>[9x]PDVPKGCEGPCKVQSYEQRHDISHVGKVLCVSDVTRGNGLTHRVGKRFCVKSVYVLGKIWMDENIKTKNHTNTVMFYLVRDRRPFGTAMDFGQVFNMYDNEPSTATIKNDLRDRYQVLRKFTSTVTGGQYASKEQALVKKFMKINNYVVYNHQEAAKYDNHTENALLLYMACTHASNPVYATLKIRIYFYDSVQN;> NRR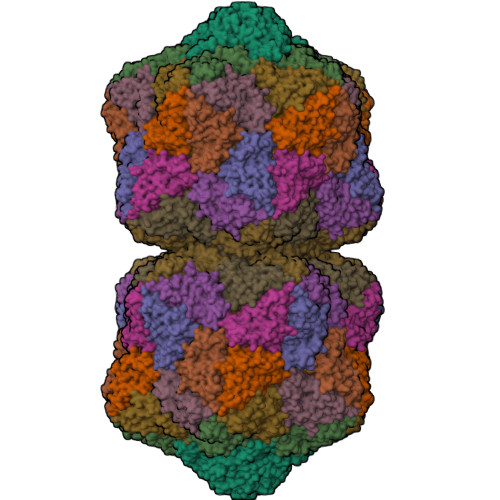RTWTNRPMYRKPRLYRMYRTPDVPKGCEGPCKVQSYEQRHDISHVGKVLCVSDVTRGNGLTHRVGKRFCVKSVYVLGKIWMDENIKTKNHTNTVMFYLVRDRRPFGTAMDFGQVFNMYDNEPSTATIKNDLRDRYQVLRKFTSTVTGGQYASKEQALVKKFMKINNYVVYNHQEAAKYDNHTENALLLYMACTHASNPVYATLKIRIYFYDSVQN;> RLYRMYRTPDVPKGCEGPCKVQSYEQRHDISHVGKVLCVSDVTRGNGLTHRVGKRFCVKSVYVLGKIWMDENIKTKNHTNTVMFYLVRDRRPFGTAMDFGQVFNMYDNEPSTATIKNDLRDRYQVLRKFTSTVTGGQYASKEQALVKKFMKINNYVVYNHQEAAKYDNHTENALLLYMACTHASNPVYATLKIRIYFYDSVQN> MTSLIDLGRYVERTHHGEDTEPRSKRVKIAKPDLSSFQPGSIIKIRLQDFVTYTLTEFNLSPSLNMIIGPNGSGKSTFVCAVCLGLAGKPEYIGRSKKVEDFIKNGQDVSKIEITLKNSPNVTDIEYIDARDETIKITRIITRSKRRSDYLINDYQVSESVVKTLVAQLNIQLDNLCQFLSQERVEEFARLKSVKLLVETIRSIDASLLDVLDELRELQGNEQSLQKDLDFKKAKIVHLRQESDKLRKSVESLRDFQNKKGEIELHSQLLPYVKVKDHKEKLNIYKEEYERAKANLRAILKDKKPFANTKKTLENQVEELTEKCSLKTDEFLKAKEKINEIFEKLNTIRDEVIKKKNQNEYYRGRTKKLQATIISTKEDFLRSQEILAQTHLPEKSVFEDIDIKRKEIINKEGEIRDLISEIDAKANAINHEMRSIQRQAESKTKSLTTTDKIGILNQDQDLKEVRDAVLMVREHPEMKDKILEPPIMTVSAINAQFAAYLAQCVDYNTSKALTVVDSDSYKLFANPILDKFKVNLRELSSADTTPPVPAETVRDLGFEGYLSDFITGDKRVMKMLCQTSKIHTIPVSRRELTPAQIKKLITPRPNGKILFKRIIHGNRLVDIKQSAYGSKQVFPTDVSIKQTNFYQGSIMSNEQKIRIENEIINLKNEYNDRKSTLDALSNQKSGYRHELSELASKNDDINREAHQLNEIRKKYTMRKSTIETLREKLDQLKREARKDVSQKIKDIDDQIQQLLLKQRHLLSKMASSMKSLKNCQKELISTQILQFEAQNMDVSMNDVIGFFNEREADLKSQYEDKKKFVKEMRDTPEFQSWMREIRSYDQDTKEKLNKVAEKYEEEGNFNLSFVQDVLDKLESEIAMVNHDESAVTILDQVTAELRELEHTVPQQSKDLETIKAKLKEDHAVLEPKLDDIVSKISARFARLFNNVGSAGAVRLEKPKDYAEWKIEIMVKFRDNAPLKKLDSHTQSGGERAVSTVLYMIALQEFTSAPFRVVDEINQGMDSRNERIVHKAMVENACAENTSQYFLITPKLLTGLHYHEKMRIHCVMAGSWIPNPSEDPKMIHFGETSNYSFD;> MISTTISGKRPIEQVDDELLSLTAQQENEEQQQQRKRRRHQFAPMTQFNSNTLDEDSGFRSSSDVATADQDNFLEESPSGYIKKVILRNFMCHEHFELELGSRLNFIVGNNGSGKSAILTAITIGLGAKASETNRGSSLKDLIREGCYSAKIILHLDNSKYGAYQQGIFGNEIIVERIIKRDGPASFSLRSENGKEISNKKKDIQTVVDYFSVPVSNPMCFLSQDAARSFLTASTSQDKYSHFMKGTLLQEITENLLYASAIHDSAQENMALHLENLKSLKAEYEDAKKLLRELNQTSDLNERKMLLQAKSLWIDVAHNTDACKNLENEISGIQQKVDEVTEKIRNRQEKIERYTSDGTTIEAQIDAKVIYVNEKDSEHQNARELLRDVKSRFEKEKSNQAEAQSNIDQGRKKVDALNKTIAHLEEELTKEMGGDKDQMRQELEQLEKANEKLREVNNSLVVSLQDVKNEERDIQHERESELRTISRSIQNKKVELQNIAKGNDTFLMNFDRNMDRLLRTIEQRKNEFETPAIGPLGSLVTIRKGFEKWTRSIQRAISSSLNAFVVSNPKDNRLFRDIMRSCGIRSNIPIVTYCLSQFDYSKGRAHGNYPTIVDALEFSKPEIECLFVDLSRIERIVLIEDKNEARNFLQRNPVNVNMALSLRDRRSGFQLSGGYRLDTVTYQDKIRLKVNSSSDNGTQYLKDLIEQETKELQNIRDRYEEKLSEVRSRLKEIDGRLKSTKNEMRKTNFRMTELKMNVGKVVDTGILNSKINERKNQEQAIASYEAAKEELGLKIEQIAQEAQPIKEQYDSTKLALVEAQDELQQLKEDINSRQSKIQKYKDDTIYYEDKKKVYLENIKKIEVNVAALKEGIQRQIQNACAFCSKERIENVDLPDTQEEIKRELDKVSRMIQKAEKSLGLSQEEVIALFEKCRNKYKEGQKKYMEIDEALNRLHNSLKARDQNYKNAEKGTCFDADMDFRASLKVRKFSGNLSFIKDTKSLEIYILTTNDEKARNVDTLSGGEKSFSQMALLLATWKPMRSRIIALDEFDVFMDQVNRKIGTTLIVKKLKDIARTQTIIITPQDIGKIADIDSSGVSIHRMRDPERQNNSNFYN;> MALNDNPIPKSVPLHPKSGKYFHNLHARDLSNIYQQCYKQIDETINQLVDSTSPSTIGIEEQVADITSTYKLLSTYESESNSFDEHIKDLK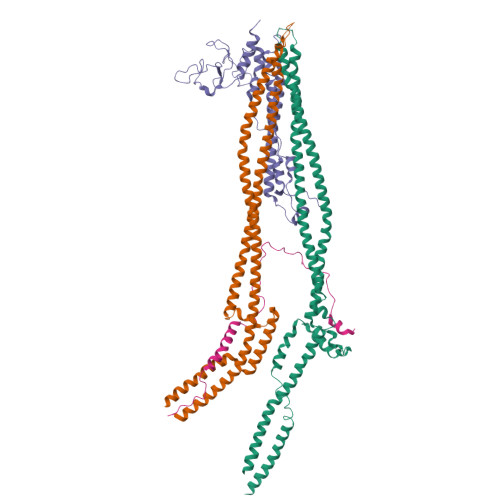KNFKQSSDACPQIDLSTWDKYRTGELTAPKLSELYLNMPTPEPATMVNNTDTLKILKVLPYIWNDPTCVIPDLQNPADEDDLQIEGGKIELTCPITCKPYEAPLISRKCNHVFDRDGIQNYLQGYTTRDCPQAACSQVVSMRDFVRDPIMELRCKIAKMKESQEQDKRSSQAIDVL;> MGSVNSSPNEEFETVPDSQISGFDSPLIPTSVGSYFRDDDDDEKVHPNFISDPENDSLNSDEEFSSLENSDLNLSGAKAESGDDFDPILKRTIISKRKAPSNNEDEEIVKTPRKLVNYVPLKIFNLGDSFDDTITTTVAKLQDLKKEILDSPRSNKSIVITSNTVAKSELQKSIKFSGSIPEIYLDVVTKETISDKYKDWHFISKNCHYEQLMDLEMKDTAYSFLFGSSRSQGKVPEFVHLKCPSITNLLVLFGVNQEKCNSLKINYEKKENSRYDNLCTIFPVNKMLKFLMYFYSDDDNDDVREFFLKAFICLILDRKVFNAMESDHRLCFKVLELFNEAHFINSYFEIVDKNDFFLHYRLLQIFPHLQSALLRRRFSEKQGRTETIQQNIIKEFNEFFDCKNYKNLLYFILTMYGSKFIPFGPKCQVTEYFKDCILDISNETTNDVEISILKGILNLFSKIR N~3~-[(2R)-2-hydroxy-4-{[(S)-hydroxy(phosphonooxy)phosphoryl]oxy}-3,3-dimethylbutanoyl]-beta-alaninamide | C9 H20 N2 O10 P2 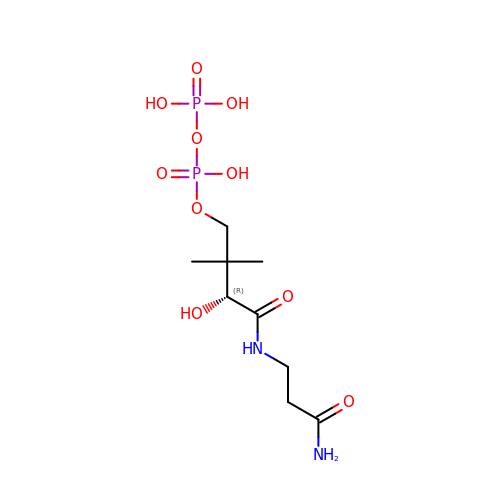| GAYRHYNVDBMBQF-ZETCQYMHSA-N{4-[4-(1,3-benzoxazol-2-yl)benzene-1-carbonyl]piperazin-1-yl}(1-hydroxycyclopropyl)methanone | C22 H21 N3 O4 | 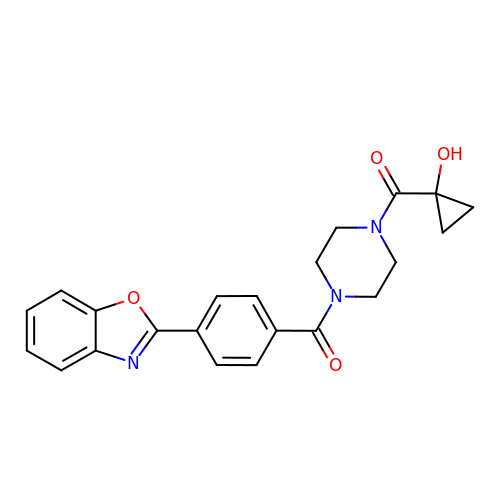FGXGECPNCZCUAJ-UHFFFAOYSA-N methyl 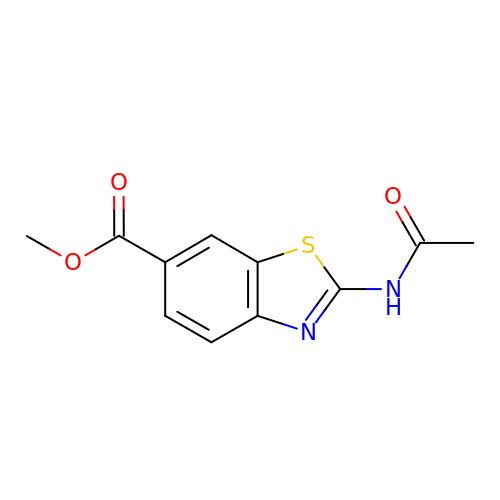2-(acetylamino)-1,3-benzothiazole-6-carboxylate | C11 H10 N2 O3 S | SJYCCQFFJCNNSS-UHFFFAOYSA-N> GQNHHEVVKFMDVYQQSYCHPIETLVDIFQEYPDEIEYIFKPSCVPLMRCGGCCNDEGLEC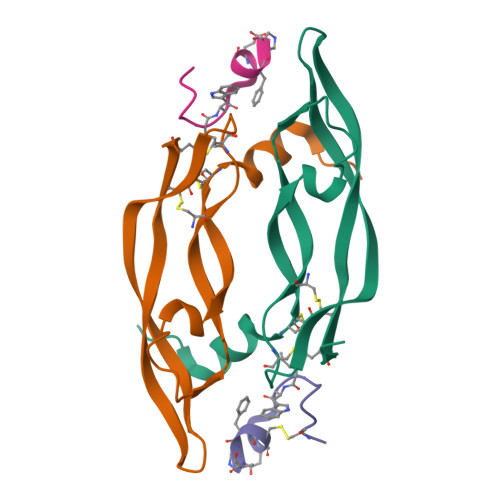VPTEESNITMQIMRIKPHQGEHIGEMSFLQHNKCECRPKAD;> GQNHHEVVKFMDVYQRSYCHPIETLVDIFQEYPDEIEYIFKPSCVPLMRCGGCCNDEGLECVPTEESNITMQIMRIKPHQGQHIGEMSFLQHNKCECRPKKD;>[2x]NCDIHVLWEWECFXR> MKLELRLKSPVGAEPAVYPWPLPVYDKHHD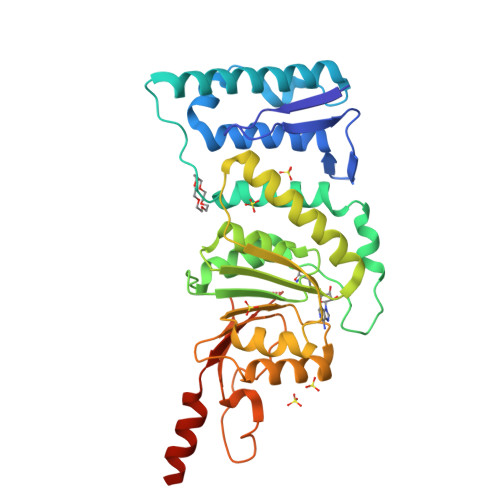AAHEIIETIRWVCEEIPDLKLAMENYVLIDYDTKSFESMQRLCDKYNRAIDSIHQLWKGTTQPMKLNTRPSTGLLRHILQQVYNHSVTDPEKLNNYEPFSPEVYGETSFDLVAQMIDEIKMTDDDLFVDLGSGVGQVVLQVAAATNCKHHYGVEKADIPAKYAETMDREFRKWMKWYGKKHAEYTLERGDFLSEEWRERIANTSVIFVNNFAFGPEVDHQLKERFANMKEGGRIVSSKPFAPLNFRINSRNLSDIGTIMRVVELSPLKGSVSWTGKPVSYYLHTIDRTILENYFSSLKLEHHHHHH> MDNSNGIHYIELTPNPIRFDAVSQLTNVFFDDSNKQIFAVRSGGATGVVVKGPGSPDDVVISFCMSDRGGAIRSIKFSPDNQILAVQRKENSVEFICFQGDQPLLQDIITHQVKTLIHGFVWVHNREVALISNTGVEVYTVVPEKRQVRSVKSLSIGIKWFAWCCDANVALLCTSEGNSLIPVLVKQKVITKLPKVDLGNPSRDVQESKVTLGQVYGVLAVLILQSNSTTGLMEVEVHLLNGPGLAPRKCHVLRLSLLGRFAINTVDNLIVVHHQASGTSLLFDISLPGEVINEITYHTPITPGRSIKPFGLKLPSLSPDGQILQCELYSTHWVLFQPNIVIDAKLGCMWFLNLCIEPLCQLISDRIRLTEFLLQRSNGKQMLLKVIGQLVDDQYKGTLLPVLETIFSRINKIYASWVQLELQNQTAQPSNVKTTTLKQSTPPIVLIEQLDMVQIFQRIARRPYTESILMLYLQSLNKFNIAAQEELSKMIISELISNRSFDTLRRLVSYSMLLESKSVACFLLSHSNVDTAISQVAIDMLGRIEAHEIIIEVMLGQGKVIDALRLAKNSMGLEKVPARKFLEAAHKTKDDLIFHSVYRFFQMRNLKLYETLSFPKAEQCTEFIQHYNNTFPADNPTRQPVS;> MAKLLQRVEITLRSFYIFNSTFGQVEGEEHKKVLFYHPNDIELNTKI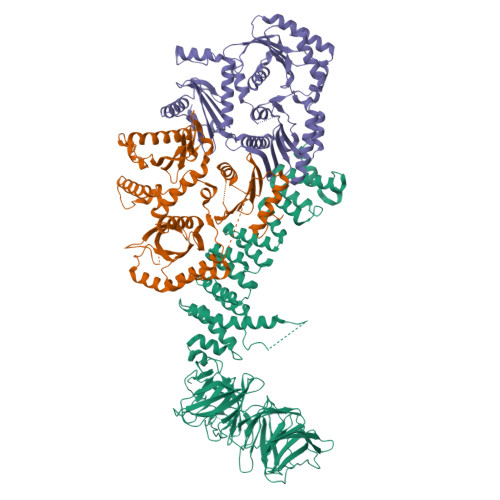KDVGLSEAIIRFTGTFTSEDDCQALHTQKTTQLFYQPEPGYWLVLVLNVPKEVRLKEGVEVADYRGAEISDRIYRAILRQCYQMFRFQNGCFSSCGSEEPNPDKRRELLCQKLLQFYDQHLTNLRDPAQCDIIDMLHSIQYLPLDKTLFLRAQNFGTLCETFPDIKESIMLYQEQVLCGGKLSPEDLHCVHSYVVQHVLKVEASSSTIAVSPSLKRSISECQVGGFVRSRQKVAGDEHDAVNEEDHPMKVYVTLDKEAKPYYLLIYRALHITLCLFLNADQVAPKQDLYDDLHAYMAPQLTSLARDISSELTKEAVGAAGQDNSSGNSETAPKYLFINEQSLQHHTNFQRHLPQGLPRNVLSIIADLANGSGKAEMESAPAEEVQVKTTNDYWIVKRRCNYRQYYVILCNSKATLLDVTQEARRIFEQELTDDVFFDKDYKDHDGDYKDHDIDYKDDDDK;> MEVEQTSVRSDTNSTCEYLDAEGDPESPNLYQEADPDQEAEQQNHSIISELRDGLGTMRDNSALSPEPGQENKGLAASVESLALSTSTSAKTEDSIGGGLEEEYDYQHDSLWQGQKKHIFILSEAGKPIFSLHGNEDKLATLFGVIQALVSFVQMGQDAITSIHAGGIKFAFMQRSSLILVAASRSNMSVQQLQLQLGDVYNQILSILTYSHMTKIFERRKNFDLRRLLSGSERLFYNLLANDSSSAKVSNNIFTFLTNSIRVFPLPTTIRSQITSAIQSNCSKIKNLVFAVLIANNKLIALVRMKKYSIHPADLRLIFNLVECSESFKSSENWSPICLPKFDMNGYLHAHVSYLADDCQACLLLLSVDRDAFFTLAEAKAKITEKLRKSHCLEAINEELQQPFNAKLYQQVVGIPELRHFLYKPKSTAQLLCPMLRHPYKSLTELERLEAIYCDLLHRIHNSSRPLKLIYEMKEREVVLAWATGTYELYAIFEPVVDKATVIKYVDKLIKWIEKEYDVYFIRNHATF> HPVEAAERNYERARAELNQANEDVARNQERQAKAVQVYNSRKSELDAANKTLADAIAEIKQFNRFAHDPMAGGHRMWQMAGLKAQRAQTDVNNKQAAFD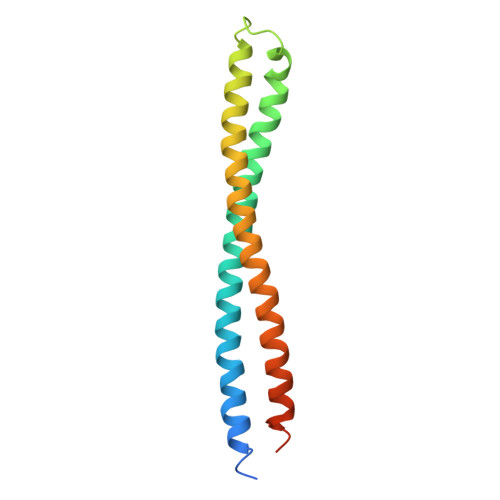AAAKEKSDADAALSSAMESRKKKEDKKRSAENNLND N-{4-[(4-hydroxy-3-nitrobenzoyl)amino]phenyl}pyridine-2-carboxamide | C19 H14 N4 O5 | 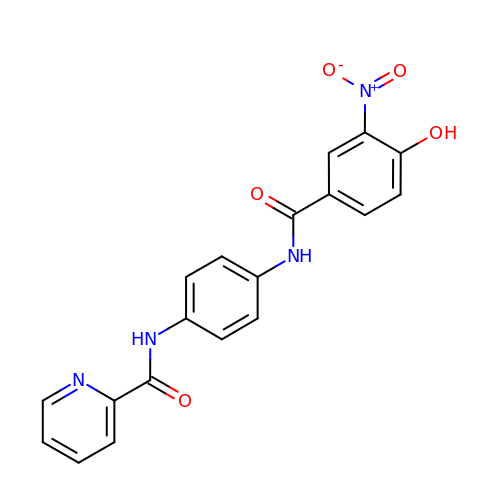QFXQBOSIGGGQEW-UHFFFAOYSA-N>SNAGKMFIGGLSWQTSPDSLRDYFSKFGEIRECMVMRDPTTKRSRGFGFVTFADPASVDKVLGQPHHELDSKTIDPKVAFPRRAQPKMVTRTKK[2x]

Musashi‐2 (MSI2) belongs to Musashi family of RNA binding proteins (RBP). Like Musashi‐1 (MSI1), it is overexpressed in a variety of cancers and is a promising therapeutic target. Both MSI proteins contain two N‐terminal RNA recognition motifs and play roles in posttranscriptional regulation of target mRNAs. Human MSI2 is a 328 amino acid protein that contains two RNA recognition motifs (RRMs) spanning G21‐K111 (RRM1) and K110‐P187 (RRM2). The C‐terminal region of MSI2 has no known motifs or specific function, while the N‐terminal RRMs mediate the binding to mRNAs,25 including those involved in the proliferation of certain cancers.

The crystal structure of MSI2‐RRM1 was modeled from residues G21 to R100 and consists of an antiparallel β‐strand core that is flanked by two α‐helices. The two subunits in the asymmetric unit form a noncrystallographic dimer in which the longest β‐stands (1, 2, 3, and 6) are positioned towards the center of the dimer. The only hydrogen bond interactions between dimer subunits occurs between residues F97/R99 in the C‐terminal β7 strand of subunit A and residues V52, M53, and R54 in β2 of subunit B. The structures of subunits A and B are quite similar with a root‐mean‐square‐deviation (RMSD) of 0.81 Å (80 residues aligned) between Cα‐atoms. A small difference between the subunits was in the loop that bridges β2 and β3. It should be noted, however, that the crystals are tightly packed as indicated by the Matthew's coefficient (Vm = 1.7 Å3/Da, 25% solvent). As such, it is possible that crystal packing could affect the conformation of the β2/β3 loop in each subunit differently. Notably, R60 in subunit A forms a contact with Q81 of a symmetry‐related molecule. However, no crystal contacts are observed with residues in the β2/β3 loop of subunit B and residues T57 and T58 were disordered. A high degree of structural similarity was observed between the crystal and solution NMR structures.> RTCRIH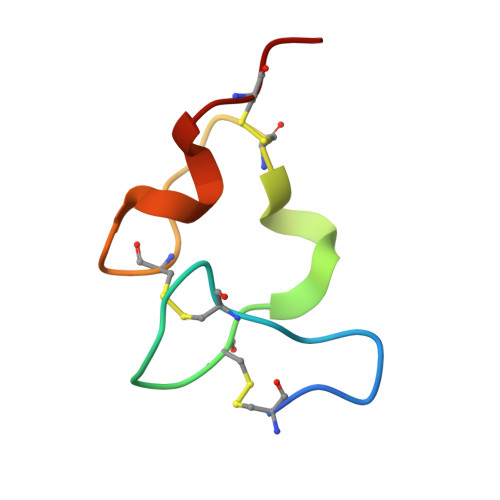EISCGAHSTQCIPVSWRCDGENDCDSGEDEENCGN>[2x]MAQYPEQLNGIFQALADPTRRAVLGRLSRGPATVSELAKPFD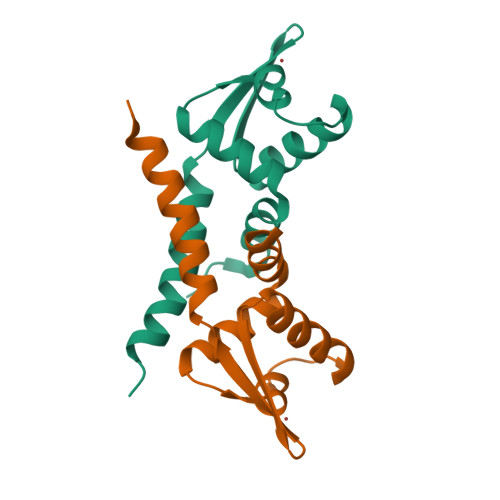MALPSFMKHIHFLEDSGWIRTHKQGRVRTCAIEKEPFTAVEAWLAEQQELWESRTDRLEQFVTEHTVTAHAKATPQ The reduction of uridine to dihydrouridine at specific positions in tRNA is catalysed by dihydrouridine synthase (Dus) enzymes. Bound FMN functions as a cofactor during the reduction of the C5—C6 double bond of uridine. Increased expression of human dihydrouridine synthase 2 (hDus2) has been linked to pulmonary carcinogenesis, while its knockdown decreased cancer cell line viability, suggesting that it may serve as a valuable target for therapeutic intervention.

Here, the X-ray crystal structure of a construct of hDus2 encompassing the catalytic and tRNA-recognition domains (residues 1–340) determined at 1.9 Å resolution is presented. It is shown that the structure can be determined automatically by phenix.mr_rosetta starting from a bacterial Dus enzyme with only 18% sequence identity and a significantly divergent structure. The overall fold of the human Dus2 is similar to that of bacterial enzymes, but has a larger recognition domain and a unique three-stranded antiparallel β-sheet insertion into the catalytic domain that packs next to the recognition domain, contributing to domain–domain interactions. The position of the recognition domain is stabilized by the three-stranded β-sheet insertion in the catalytic domain, which packs next to the recognition domain. Interactions between the extended C-terminal helix of the recognition domain and the three-stranded β-sheet of the catalytic domain that were not seen in bacterial Dus enzymes appear to extend the domain interface and may stabilize the overall structure. Density-modified SAD phases resulted in clear electron-density maps and autobuilding was able to produce an almost complete model. The FMN density was nonplanar, hence the two-electron-reduced form (PDB ligand ID FNR) was used during the refinement. Part of the positively charged and conserved area of hDus2 corresponds to the active site containing the bound FMN molecule. The corresponding segment of hDus2 (residues 118–128) is not defined in the electron-density maps. Conservation of the catalytic residues indicates that the enzymatic mechanism is essentially the same as for the bacterial homologues. We propose that structural differences and differences in the electrostatic surface may result in altered positioning of tRNA during catalysis compared with bacterial enzymes.

> GSHMASMILNSLSLCYHNKLILAPMVRVGTLPMRLLALDYGADIVYCEELIDLKMIQCKRVVNEVLSTVDFVAPDDRVVFRTCEREQNRVVFQMGTSDAERALAVARLVENDVAGIDVNMGCPKQYSTKGGMGAALLSDPDKIEKILSTLVKGTRRPVTCKIRILPSLEDTLSLVKRIERTGIAAIAVHGRKREERPQHPVSCEVIKAIADTLSIPVIANGGSHDHIQQYSDIEDFRQATAASSVMVARAAMWNPSIFLKEGLRPLEEVMQKYIRYAVQYDNHYTNTKYCLCQMLREQLESPQGRLLHAAQSSREICEAFGLGAFYEETTQELDAQQARLSAKTSE> GSQNLDSMLHGTGMKSDSDQKKSENGVTLAPEDTLPFLKCYCSGHCPDDAINNTCITNGHCFAIIEEDDQGETTLASGCMKYEGSDFQCKDS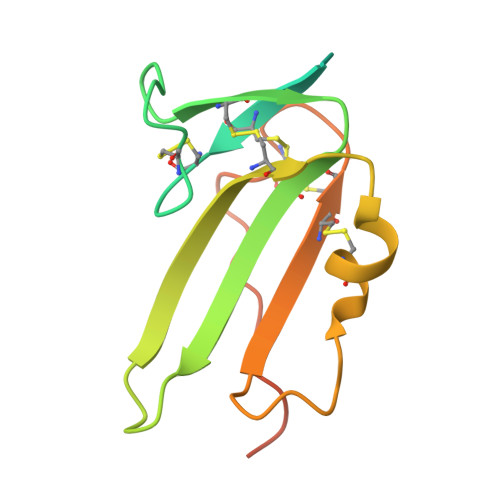PKAQLRRTIECCRTNLCNQYLQPTLPPVVIGPFFDGSIR> MEKMSSGTPTPSNVVLIGKKPVMNYVLAALTLLNQGVSEIVIK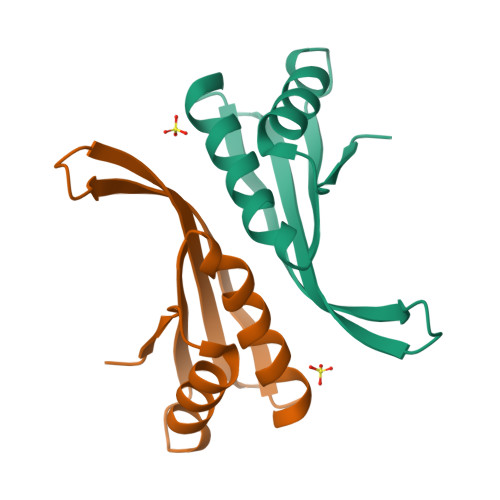ARGRAISKAVDTVEIVRNRFLPDKIEIKEIRVGSQVVTSQDGRQSRVSTIEIAIRKK>[3x]MEYKSSPKRPYLLRAYYDWLVDNSFTPYLVVDATYLGVNVPVEYVKDGQIVLNLSASATGNLQLTNDFIQFNARF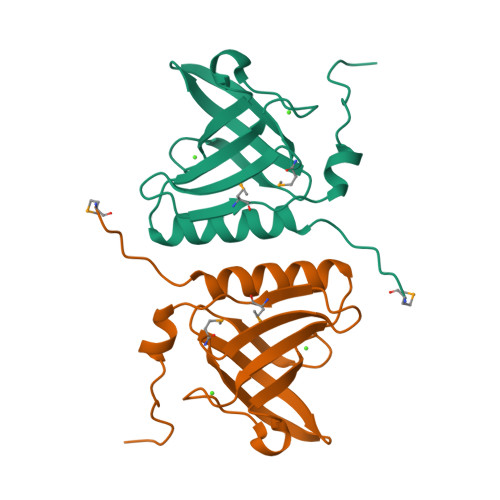KGVSRELYIPMGAALAIYARENGDGVMFEPEEIYDELNIEPDTEQPTGFYEAVD>GPLGSMPGEEEERAFLVAREELASALRRDSGQAFSLEQLRPLLASSLPLAARYLQLDAARLVRCNAHGEPRNYLNTLSTALNILEKYGRNLLSPQRPRYWRGVKFNNPVFRSTVDAVQGGRDVLRLYGYTEEQPDGLSFPEGQEEPDEHQVATVTLEVLLLRTELSLLLQNTHPR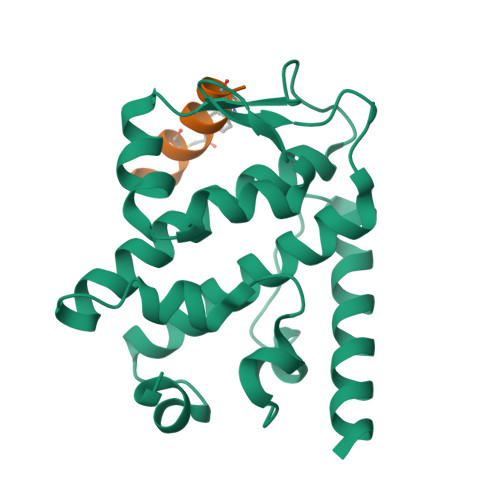QQALEQLLE[2x];>FTDCQLAAAVCMTY[2x]> HG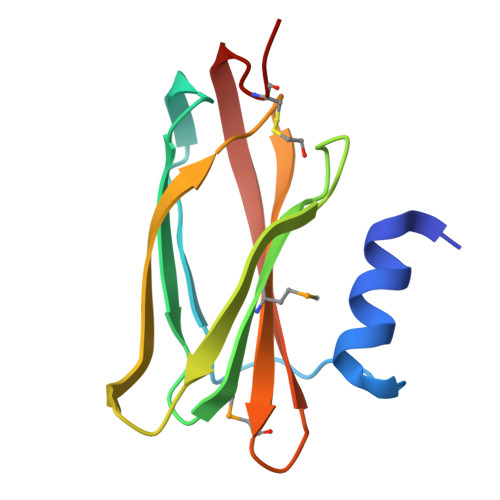SSTVDELTAAFTGGAATGEGGLTLTAPEIAENGNTVPIEVKAPGAVAIMLLAAGNPEPAVATFNFGPAAADQRAATRIRLAQTQDVIALAKMADGSVVKAQTTVKVTIGGCGG> FTETTIVVHYHRYDGKYDGWNLWIWPVEPVSQEGKAYQFTGEDDFGKVAVVKLPMDLTKVGIIVRLNEWQAKDVAKDRFIEIKDGKAEVWILQGVEEIFY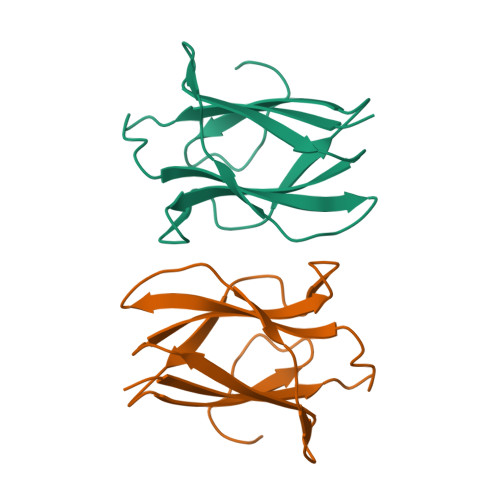EKP>GSAGAGAMTIVNRIRTDVVNVAKSFGAEYSEAVIDQIFQGFGEKFTNTGFAIRVQNKRNQKVDCNIRYGEAKENCLAWDIARESGLLSDQGHPVDTLIQEMFQAIPAIAYGADFDINYGLVKIWHLPKIVPVEEAFKIPSLPKSVNAHIDFFKKYHLDALCALTVDYRNKSTNLYFDAHHPEQRTTQFYKNILQSQQFEVPSDEVLEILVNCPEIAVTFNWSSPGIERMCFYTAFVNRETVPQHINPVLKKFAQEAPALLDNPGFLVGWSFGPDAKKGTYIKIDVDYHGLVV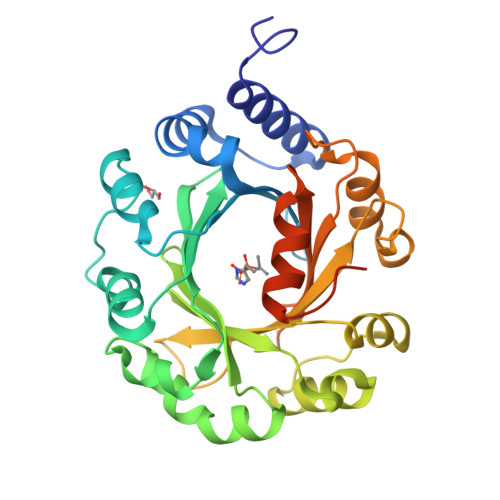PSFFHMHNLPLPIPEANSVFDLPSSDTEDKLNSIVMS[2x]In this work, we report the first SSX experiments with viscous jets conducted at ALBA beamline BL13-XALOC. Small crystals (15–30 µm) of five soluble proteins (lysozyme, proteinase K, phycocyanin, insulin and α-spectrin-SH3 domain) were suspended in lipidic cubic phase (LCP) and delivered to the X-ray beam with a high-viscosity injector developed at Arizona State University. Complete data sets were collected from all proteins and their high-resolution structures determined. The high quality of the diffraction data collected from all five samples, and the lack of specific radiation damage in the structures obtained in this study, confirm that the current capabilities at the beamline enables atomic resolution determination of protein structures from microcrystals as small as 15 µm using viscous jets at room tem­per­ature.

In addition to the standard model system, i.e. proteins such as hen egg-white lysozyme and proteinase K from Tritirachium album limber, we included phycocyanin from Thermosynechococcus elongatus, human insulin and the SH3 domain of α-spectrin (α-spectrin-SH3) from Gallus gallus.

> AAQTNAPWGLARISSTSPGTSTYYYDESAGQGSCVYVIDTGIEASHPEFEGRAQMVKTYYYSSRDGNGHGTHCAGTVGSRTYGVAKKTQLFGVKVLDDNGSGQYSTIIAGMDFVASDKNNRNCPKGVVASLSLGGGYSSSVNSAAARLQSSGVMVAVAAGNNNADARNYSPASEPSVCTVGASDRYDRRSSFSNYGSVLDIFGPGTDILSTWIGGSTRSISGTSMATPHVAGLAAYLMTLGKTTAASACRYIADTANKGDLSNIPFGTVNLLAYNNYQA>SMNFYSAYQHGFVRVAACTHHTTIGDPAANAASVLDMARACHDDGAALAVFPELTLSGYSIEDVLLQDSLLDAVEDALLDLVTESADLLPVLVVGAPLRHRHRIYNTAVVIHRGAVLGVVPKSYLPTYREFYERRQMAPGDGERGTIRIGGADVAFGTDLLFAASDLPGFVLHVEIAEDMFVPMPPSAEAALAGATVLANLSGSPITIGRAEDRRLLARSASARCLAAYVYAAAGEGESTTDLAWDGQTMIWENGALLAESERFPKGVRRSVADVDTELLRSERLRMGTFDDNRRHHRELTESFRRIDFALDPPAGDIGLLREVERFPFVPADPQRLQQDCYEAYNIQVSGLEQRLRALDYPKVVIGVSGGLDSTHALIVATHAMDREGRPRSDILAFALPGFATGEHTKNNAIKLARALGVTFSEIDIGDTARLMLHTIGHPYSVGEKVYDVTFENVQAGLRTDYLFRIANQRGGIVLGTGDLSELALGWSTYGVGDQMSHYNVNAGVPKTLIQHLIRWVISAGEFGEKVGEVLQSVLDTEITPELIPTGEEELQSSEAKVGPFALQDF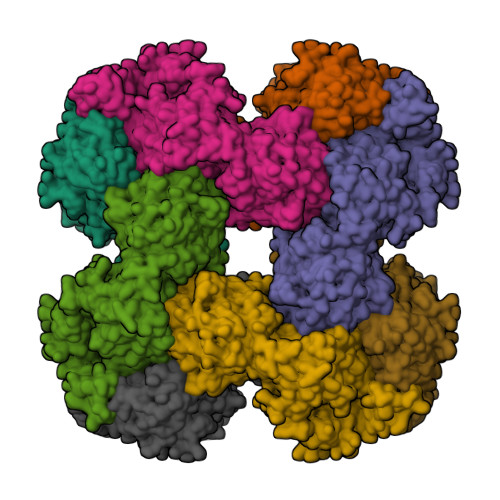SLFQVLRYGFRPSKIAFLAWHAWNDAERGNWPPGFPKSERPSYSLAEIRHWLQIFVQRFYSFSQFKRSALPNGPKVSHGGALSPRGDWRAPSDMSARIWLDQIDREVPKG[4x]> MSLADISVIQSLPLSGSQAVTGRALNAGARLYFDWLNLNGGINGETIRLVARDDEQKIEQTVRNVRDMARVDNPVALLTVVGTANVEALMREGVLAEAR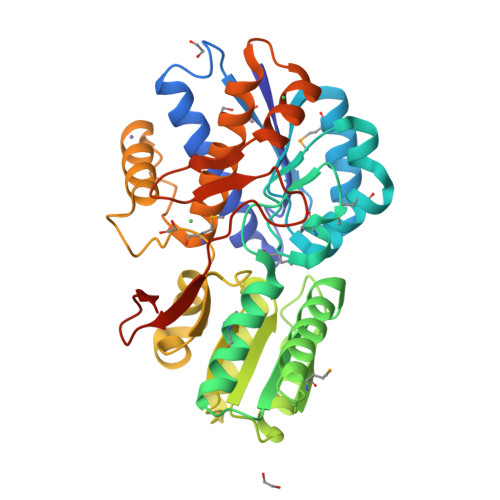LPLVGPATGASSMTTDPLVFPIKASYQQEIDKMITALVTIGVTRIGVLYQEDALGKEAITGVERTLKAHALAITAMASYPRNTANVGPAVDKLLAADVQAIFLGATAEPAAQFVRQYRARGGEAQLLGLSSIDPGILQKVAGLDAVRGYSLALVMPNPGKSVNPVIREFNRARAAVGAKDVDLSFRAVEGFVAAKVLAEAIRRAGPKPTREQVRHALTELRDYDVGGGFTVDFTDRSRPGSHYIELGVVGPNGLVIQEGHHHHHH>HPETLVKVKDAEDQLGARVGYIELDLNSGKILESFRPEERFPMMSTFKVLLCGAVLSRVDAGQEQLGRRIHYSQNDLVEYSPVTEKHLTDGMTVRELCSAAITMSDNTAANLLLTTIGGPKELTAFLHNMGDHVTRLDRWEPELNEAIPNDERDTTMPAAMATTLRKLLTGELLTLASRQQLIDWMEADKVAGPLLRSALPAGWFIADKSGAGERGSRGIIAALGPDGKPSRIVVIYTTGSQATMDERNRQIAEIGASLIKHW[2x];>[2x]AGVMTGAKFTQIQFGMTRQQVLDIAGAENCETGGSFGDSIHCRGHAAGDYYAYATFGFTSAAADAKVDSKSQEKLLAPSAPTLTLAKFNQVTVGMTRAQVLATVGQGSCTTWSEY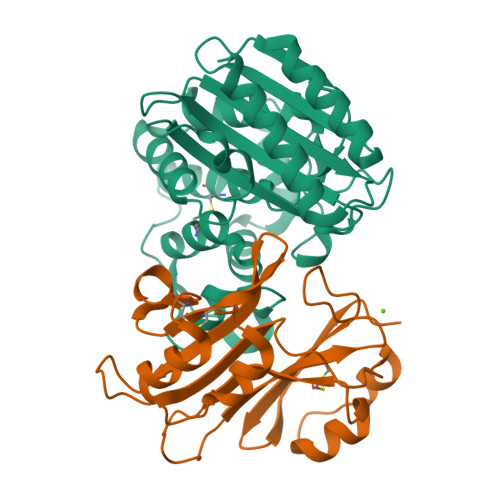YPAYPSTAGVTLSLSCFDVDGYSSTGAYRGSAHLWFTDGVLQGKRQWDLV(5-methoxy-1H-indol-3-yl)acetic acid | C11 H11 N O3 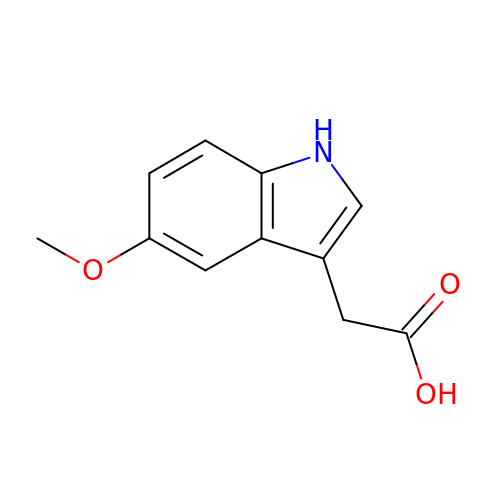| COCNDHOPIHDTHK-UHFFFAOYSA-N>NSIIGEKYRWPHTIPYVLEDSLEMNAKGVILNAFERYRLKTCIDFKPWAGETNYISVFKGS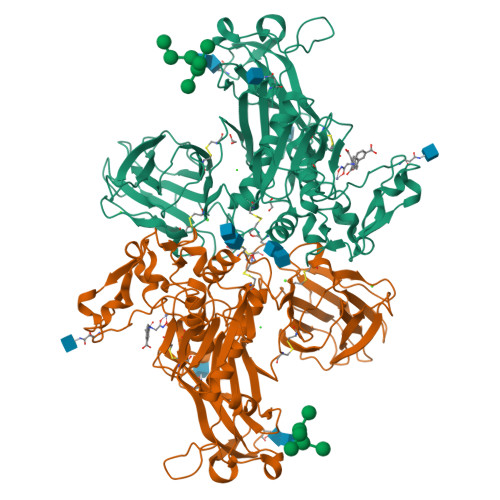GCWSSVGNRRVGKQELSIGANCDRIATVQHEFLHALGFWHEQSRSDRDDYVRIMWDRILSGREHNFNTYSDDISDSLNVPYDYTSVMHYSKTAFQNGTEPTIVTRISDFEDVIGQRMDFSDSDLLKLNQLYNCSSSLSFMDSCSFELENVCGMIQSSGDNADWQRVSQVPRGPESDHSNMGQCQGSGFFMHFDSSSVNVGATAVLESRTLYPKRGFQCLQFYLYNSGSESDQLNIYIREYSADNVDGNLTLVEEIKEIPTGSWQLYHVTLKVTKKFRVVFEGRKGSGASLGGLSIDDINLSETRCPHHIWHIRNFTQFIGSPNGTLYSPPFYSSKGYAFQIYLNLAHVTNAGIYFHLISGANDDQLQWPCPWQQATMTLLDQNPDIRQRMSNQRSITTDPFMTTDNGNYFWDRPSKVGTVALFSNGTQFRRGGGYGTSAFITHERLKSRDFIKGDDVYILLTVEDISHLNSTQ[2x]Transporters of the Nramp (Natural resistance-associated macrophage protein) family import divalent transition metal ions into cells of most organisms. In addition to the physiological substrates Fe2+ and Mn2+, Nramps can also transport toxic metals like Cd2+ and Hg2+ but exclude the abundant alkaline earth metals like Mg2+ and Ca2+. Recent bacterial Nramp structures reveal a LeuT fold, three stable conformations (outward-open, occluded, and inward-open), and identify the metal-binding site residues, including conserved aspartate, asparagine, and methionine residues. We present high-resolution structures of DraNramp in three conformations in both Mn2+-bound and metal-free states, providing the first molecular map of the entire Mn2+ transport cycle.

Two new structures of DraNramp point-mutants reveal the coordination of Mn2+ in the inward-open state: M230A•Mn2+ and D296A•Mn2+ (Cα RMSD of 0.42 Å). As in the occluded state, the Mn2+ binds D56, N59, and the A227 carbonyl, with a water replacing M230 in M230A•Mn2+. However, with TM1a displaced, the A53 carbonyl no longer coordinates Mn2+; instead, the Y54 carbonyl approaches Mn2+ at a longer distance of 3.1 Å. Two more waters, one bound to Q378 and another from the inner vestibule, complete a seven-coordination sphere resembling a pentagonal bipyramidal geometry with substantial distortion. Seven coordination is infrequent but found in Mn2+-coordinating proteins like MntR. TM1a swings to a similar angle in the new inward-open M230A•Mn2+ as in the previous low-resolution inward-open metal-free structure, and structures of the homologous Eggerthella lenta Nramp-related magnesium transporter (EleNRMT), LeuT, and serotonin transporter. However, in M230A•Mn2+ H232 flips to interact with the G330 carbonyl (TM8), suggesting that it may transiently move during the conformational cycle. Mn2+ is present at the external site in the inward-open M230A•Mn2+, and consistently, the ITC data fit a two-site model (Kd1=215±65 µM assigned to the orthosteric site, Kd2=4600±1300 µM for the external site). M230 is thus a crucial ligand for Cd2+ but not Mn2+, which is further reflected in the transport behavior where M230A affects Cd2+ transport drastically but has negligible effect on Mn2+. The occluded and inward-open states may be energetically similar as relatively small perturbations yielded inward-open structures (M230A•Mn2+ and D296A•Mn2+).

> MHHHHHHHHAGPRGVRRILPFLGPAVIASIAYMDPGNFATNIEGGARYGYSLLWVILAANLMAMVIQNLSANLGIASGRNLPELIRERWPRPLVWFYWIQAELVAMATDLAEFLGAALAIQLLTGLPMFWGAVVTGVVTFWLLNLQKRGTRPLELAVGAFVLMIGVAYLVQVVLARPDLAAVGAGFVPRLQGPGSAYLAVGIIGATVAPHVIYLHSALTQGRIQTDTTEEKRRLVRLNRVDVIAAMGLAGLINMSMLAVAAATFHGKNVENAGDLTTAYQTLTPLLGPAASVLFAVALLASGLSSSAVGTMAGDVIMQGFMGFHIPLWLRRLITMLPAFIVILLGMDPSSVLILSQVILCFGVPFALVPLLLFTARRDVMGALVTRRSFTVIGWVIAVIIIALNGYLLWELLGG>MTFEIVFDSAREFESLIATLEKFFDEAVFQVNMEGIQMRAIDPSRVVLVDLNLPEMLFSKYSVESEEAIAFDLKRFLKVLKLARSRDTLVLRKGGENFLEVGLLGDENTWFKLPLIDANTPEIEIPSLPWTVKAVVLAGALKRAVKAAKLVSDSIYFMATPEKLTFKAEGNDSEVRTVLTMEDPGLLDLEHKMTKAKSAYGVAYLEDILRSLADADEVIIRFGFDIPLLLKYMVRDAGEVSFLIAPRVEEG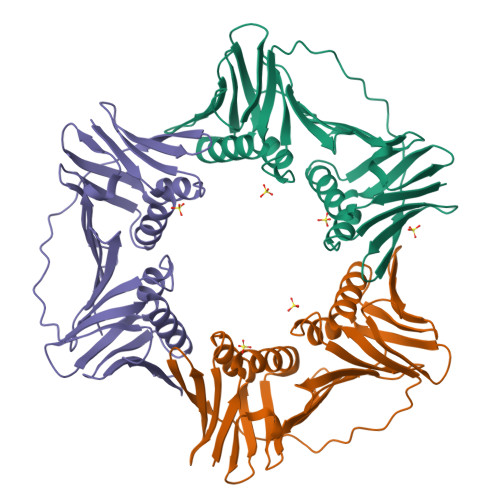RSHHHHHH[3x]> ALVKEEIQAKEYLENLNKELAKRTNVETEAAWAYGSNITDENEKKKNEISAELAKFMKEVASDTTKFQWRSYQSEDLKRQFKALTKLGYAALPEDDYAELLDTLSAMESNFAKVKVCDYKDSTKCDLALDPEIEEVISKSRDHEELAYYWREFYDKAGTAVRSQFERYVELNTKAAKLNNFTSGAEAWLDEYEDDTFEQQLEDIFADIRPLYQQIHGYVRFRLRKHYGDAVVSETGPIPMHLLGNMWAQQWSEIADIVSPFPEKPLVDVSAEMEKQGYTPLKMFQMGDDFFTSMNLTKLPQDFWDKSIIEKPTDGRDLVCHASAWDFYLIDDVRIKQCTRVTQDQLFTVHHELGHIQYFLQYQHQPFVYRTGANPGFHEAVGDVLSLSVSTPKHLEKIGLLKDYVRDDEARINQLFLTALDKIVFLPFAFTMDKYRWSLFRGEVDKANWNCAFWKLRDEYSGIEPPVVRSEKDFDAPAKYHISADVEYLRYLVSFIIQFQFYKSACIKAGQYDPDNVELPLDNCDIYGSAAAGAAFHNMLSMGASKPWPDALEAFNGERIMSGKAIAEYFEPLRVWLEAENIKNNVHIGWTTSNKCVS;>RW[2x]

Angiotensin-I-converting enzyme (ACE, EC 3.4.15.1) is a promiscuous zinc metallopeptidase with a number of substrates, including the vasoregulatory peptides angiotensin I and bradykinin, the anti-fibrotic agent N-acetyl-SDKP, the neurotransmitter substance P, and amyloid-β peptide. Here, we present the use of the Drosophila melanogaster ACE homologue, AnCE (which, in particular, shares enzymatic properties with cACE), as a model to study the structural basis of ACE inhibition. The active site is located at the centre of this channel, marked by the location of the catalytic zinc ion, which is coordinated by His367, His371, and Glu395. The high-resolution crystal structures of AnCE in complex with the dipeptides VW, IW, YW, RW, and WR presented here reveal dual binding in both the non-prime (dipeptide-1) and prime (dipeptide-2) subsites of AnCE.

The RW-1 arginine shows significantly more interactions when compared to IW-1 isoleucine and VW-1 valine; this is likely due to a much larger charged side chain, resulting in it being able to interact with more distant residues. The arginine interacts with the S1 subsite residues mostly through water-mediated interactions, with the exception of the arginine side chain directly forming H-bonds with Tyr496 (also observed in YW) and a salt bridge with Glu124 (which has moved relative to Glu124 in native AnCE). The side chain further interacts with the following S1 residues through a series of water-mediated interactions: Ala47, Lys62, Ser339, Lys352, Ala500, and Asp501, as well as His337 from the S1′ subsite. The RW-2 arginine side chain forms the most interactions out of all the dipeptides listed in this section. The side chain forms H-bonds with Gln266 and Thr364 and water-mediated interactions with Glu150, Asn261, Gln265, and Gln361. The arginine also forms a salt bridge with Asp360 and hydrophobic contacts with Ala338 and Thr364. RW-2 tryptophan is positioned towards the S2′ subsite, and the arginine sits within S1′, but in WR-2, the opposite is true. The difference in orientation between RW and WR likely favours RW binding due to the tryptophan occupying the more hydrophobic S2 and S2′ subsites. Interestingly, RW has a Ki value of 200 µM (0.2 mM), showing a significantly tighter binding when compared to WR (840 µM). The favourability in this orientation of binding is also shown by RW having a higher affinity for AnCE than WR (200 µM and 840 µM, respectively).>[6x]ADSVNGAK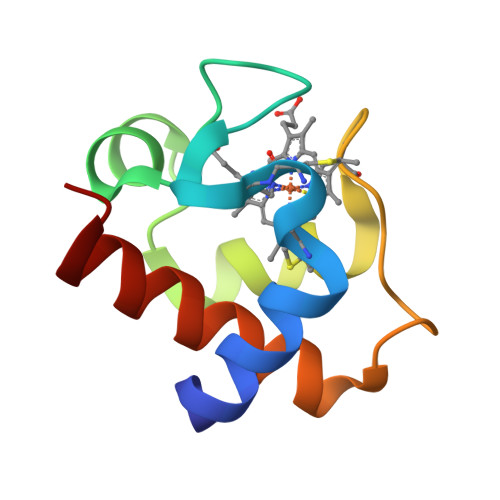IFSANCASCHAGGKNLVQAQKTLKKADLEKYGMYSAEAIIAQVTNGKNAMPAFKGRLKPEQIEDVAAYVLGKADADWK> MALDLTGYLDRINYRGATDPTLDVLRDLVSAHTGAIAFENLDPLMGVPVDDLSAEALADKLVDRRRGGYCYEHNGLIGYVLAELGYRVRRLAGRVVWLAPPDAPTPAQTHTVLAVTFPGCQGPYLVDVGFGGMTPTAPLRLETGTV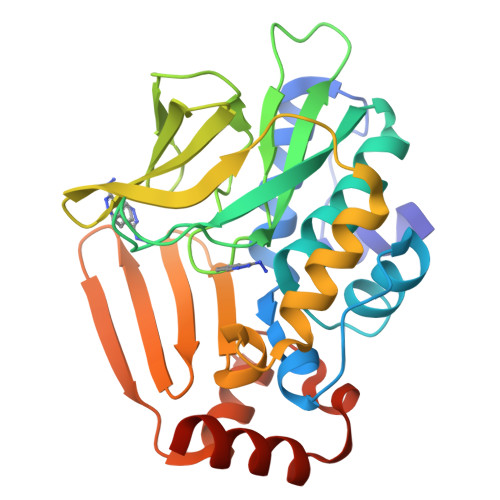QQTALEPYRLDDRGDGLVLQAMVRDEWQALYEFSTLTRPQVDLRVGSWFVSTHPTSHFVTGLMAATVADDARWNLMGRNLAIHRRGGTEKILLEDAAAVVDTLGDRFGINVADVGERGRLEARIDKVCFGAENR>[2x]APAAVDWRARGAVTAVKDQGQCGSCWAFSAIGNVECQWFLAGHPLTNLSEQMLVSCDKTDSGCSGGLMNNAFEWIVQENNGAVYTEDSYPYASGEGISPPCTTSGHTVGATITGHVELPQDEAQIAAWLAVNGPVAVAVDASSWMTYTGGVMTSCVSEQLDHGVLLVGYNDSAAVPYWIIKNSWTTQWGEEGYIRIAKGSNQCLVKEEASSAVVG

The major cysteine protease of T. cruzi, cruzain, is an attractive target for the development of trypanocidal agents. Cruzain is expressed throughout the parasite life cycle and plays important roles in the survival of the organism, including immunoevasion, acquisition of nutrients, and parasite differentiation. X-ray crystal structures of cruzain in complex with reversible, [11]and irreversible inhibitors have been reported, and the overall folding pattern and structure of the active site is highly homologous to papain. Seven substrate binding sites, four (S4, S3, S2, and S1) on the acyl side and three (S1′, S2′, and S3′) on the amino side of the scissile bond, form a cleft between two structural domains of the enzyme.

The catalytic triad of Cys25, His159, and Asn175, as well as the highly conserved Trp177, is contained within this cleft. Like most other papain-like cysteine proteases, the interaction of the S2 site of the enzyme with the complementary P2 residue is the key specificity determining factor. Cruzain is able to accommodate phenylalanine or arginine in the P2 position of the ligand due to the presence of Glu208 (cruzain numbering) found at the base of the S2 pocket, which can form a salt bridge with the positively charged arginine side chain. [24]The vinyl sulfone warhead acts as a Michael acceptor for the active site Cys25, while the sulfone unit and the peptide framework provide several hydrogen bond acceptors that interact favorably with complementary residues in the active site. In recent years, K11777 (1), a selective cruzain inhibitor, has been demonstrated to eradicate T. cruzi infection in cell culture, mouse, and dog models. To date, all of our compounds contain a hydrophobic group at the P2 site. Herein, we report the synthesis of WRR-483 (2), the arginine variant of K11777, its remarkable biological properties, and a crystal structure of WRR-483 bound to cruzain.> MKTMRKQIYKKAYWLLLPFLPLALANTFLVKEDSKNVTAYTPFATPITDSKSDLVSLAQLDSSYQIADQTIHNTNLFVLFKSRDVKVKYESSGSNNISFDSTSQGEKPSYVVEFTNSTNIGIKWTMVKKYQLDVPNVSSDMNQVLKNLILEQPLTKYTLNSSLAKEKGKTQREVHLGSGQANQWTSQRNQHDLNNNPSPNASTGFKLTTGNAYRKLSESWPIYEPIDGTKQGKGKDSSGWSSTEENEAKNDAPSVSGGGSSSGTFNKYLNTKQALESIGILFDDQTPRNVITQLYYASTSKLAVTNNHIVVMGNSFLPSMWYWVVERSAQENASNKPTWFANTNLDWGEDKQKQFVENQLGYKETTSTNSHNFHSKSFTQPAYLISGIDSVNDQIIFSGFKAGSVGYDSSSSSSSSSSSSTKDQALAWSTTTSLDSKTGYKDLVTNDTGLNGPINGSFSIQDTFSFVVPYSGNHTNNGTTGPIKTAYPVKKDQKSTVKINSLINATPLNSYGDEGIGVFDALGLNYNFKSNQERLPSRTDQIFVYGIVSPNELRSAKSSADSTGSDTKVNWSNTQSRYLPVPYNYSEGIIDADGFKRPENRGASVTTFSGLKSIAPDGFANSIANFSVGLKAGIDPNPVMSGKKANYGAVVLTRGGVVRLNFNPGNDSLLSTTDNNIAPISFSFTPFTAAESAVDLTTFKEVTYNQESGL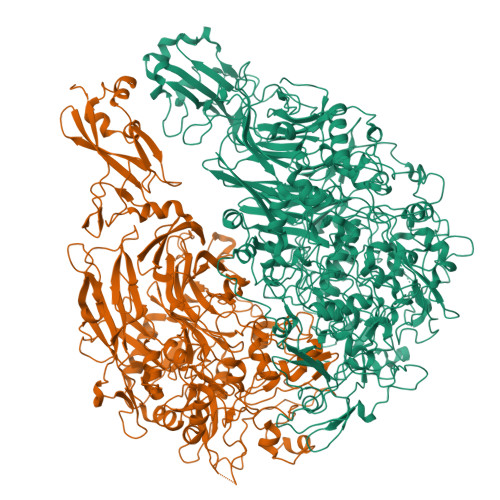WSYIFDSSLKPSHDGKQTPVTDNMGFSVITVSRTGIELNQDQATTTLDVAPSALAVQSGIQSTTQTLTGVLPLSEEFSAVIAKDSDQNKIDIYKNNNGLFEIDTQLSNSVATNNGGLAPSYTENRVDAWGKVEFADNSVLQARNLVDKTVDEIINTPEILNSFFRFTPAFEDQKATLVATKQSDTSLSVSPRIQFLDGNFYDLNSTIAGVPLNIGFPSRVFAGFAALPAWVIPVSVGSSVGILFILLVLGLGIGIPMYRVRKLQDASFVNVFKKVDTLTTAVGSVYKKIITQTGVVKKAPSALKAANPSVKKPAAFLKPPVQPPSKPEGEQKAVEVKSEETKS;> MHQPKKRLAKKSWAFLTAALTLGVITGVGGYFLFNQNKQRSSVSNFAYQPKQLSVKHQQAVDETLTPWTWNNNNFSSLKITGENPGSFGLVRSQNDNLNISSVTKNSSDDNLKYLNAVEKYLDGQQNFAIRRYDNNGRALYDINLAKMENPSTVQRGLNGEPIFDPFKGFGLTGNAPTDWNEIKGKVPVEVVQSPHSPNLYFVLLVPKVALEYHNLNNQVVKESLEVKATQSSFNPTQRLQKDSPVKDSSKQGEKLSETTASSMSSGMATSTRAKALKVEVERGSQSDSLLKNDFAKKPLKHKNSSGEVKLEAEKEFTEAWKPLLTTDQIAREKGMGATVVSFYDAPYSENHTAFGLVDHIDPKKMVENYPPSWKTPKWNHHGIWDYNARNLLLQTTGFFNPRRHPEWFDEGQAKADNTSPGFKVGDTDHKKDGFKKNSSSPIALPFEAYFANIGNMVAIGNSVFIFGGNGHATKMFTTNPLSIGVFRIKYTDNFSKSSVTGWPYAVLFGGLINPQTNGLKDLPLGTNRWFEYVPRMAVSGVKWVGNQLVLAGTLTMGDTATVPRLKYDQLEKHLNLVAQGQGLLREDLQIFTPYGWANRPDIPVGAWLQDEMGSKFGPHYFLNNPDIQDNVNNDTVEALISSYKNTDKLKHVYPYRYSGLYAWQLFNWSNKLTNTPLSANFVNENSYAPNSLFAAILNEDLLTGLSDKIFYGKENEFAENEADRFNQLLSLNPNPNTNWARYLNVVQRFTTGPNLDSSTFDQFLDFLPWIGNGKPFSNSPSPSTSASSSTPLPTFSNINVGVKSMITQHLNKENTRWVFIPNFSPDIWTGAGYRVQSANQKNGIPFEQVKPSNNSTPFDPNSDDNKVTPSGGSSKPTTYPALPNSISPTSDWINALTFTNKNNPQRNQLLLRSLLGTIPVLINKSGDSNDQFNKDSEQKWDKTETNEGNLPGFGEVNGLYNAALLHTYGFFGTNTNSTDPKIGFKADSSSSSSSTLVGSGLNWTSQDVGNLVVINDTSFGFQLGGWFITFTDFIRPRTGYLGITLSSLQDQTIIWADQPWTSFKGSYLDSDGTPKSLWDPTALKSLPNSSTTYDTNPTLSPSFQLYQPNKVKAYQTTNTYNKLIEPVDATSAATNMTSLLKLLTTKNIKAKLGKGTASSQGNNNGGGVSQTINTITTTGNISEGLKEETSIQAETLKKFFDSKQNNKSEIGIGDSTFTKMDGKLTGVVSTPLVNLINGQGATSDSDTEKISFKPGNQIDFNRLFTLPVTELFDPNTMFVYDQYVPLLVNLPSGFDQASIRLKVISYSVENQTLGVRLEFKDPQTQQFIPVLNASSTGPQTVFQPFNQWADYVLPLIVTVPIVVIILSVTLGLTIGIPMHRNKKALQAGFDLSNKKVDVLTKAVGSVFKEIINRTGISNAPKKLKQATPTKPTPKTPPKPPVKQ> GSFLPNSEQQKSVDIVFSSPQDL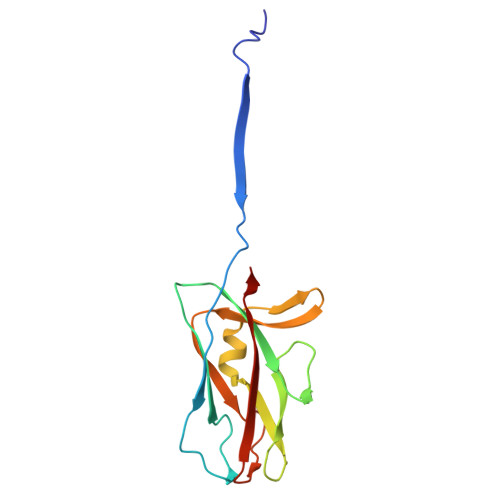TVSLIPVSGLKAGKNAPSAKIAKLVVNSTTLKEFGVRGISNNVVDSTGTAWRVAGKNTGKEIGVGLSSDSLRRSDSTEKWNGVNWMTFNSNDTLDIVLTGPAQNVTADTYPITLDVVGYQP> QGMTETISTPAATTTPDLADQQELERRVAQVVSNDPQLQALLPDDAVSGAVNEPGLTLIELIRRLLEGYGDRPALGQRAVELVTDEHGATTVALKTEFVTTSYRELWNRAEAIAAAWYAQGIRDGDFVAQLGFTSTDFASLDVAGLRLGTVSVPLQTGASVQQRNAILEETQPTVFAASVEYLEAAVDSVLATPSVQLLSVFDYHPEADAHRAALSAVRDRLETAGRTITIDSLGDAIARGRELPAAPQPSEDPDALRLLIYTSGSTGTPKGAMYPQWLVANLWQKKWLTTTVIPSVGVNFMPMSHLAGRLTLMGTLSGGGTAYYIASSDLSTFFEDIALIRPTEVLFVPRVVEMVFQRYQAELDRSLAPGESNAEIAEKIKVRIREEDFGGRVLNAGSGSAPLSPEMNDFMESLLQVAMLDGYGSTEAGAVWRDGVLQRPPVTEYKLVDVPELGYFTTDSPHPRGELRIKSETMFPGYYKRPETTADVFDEDGFYMTGDVVAELGPDHLKYLDRVKNVLKLAQGEFVAVSKLEAAYTGSPLVRQIFVYGNSERSYLLAVVVPTPEALERYADSPDALKPLIQDSLQQVAKGAELQSYEIPRDFIVETVPFT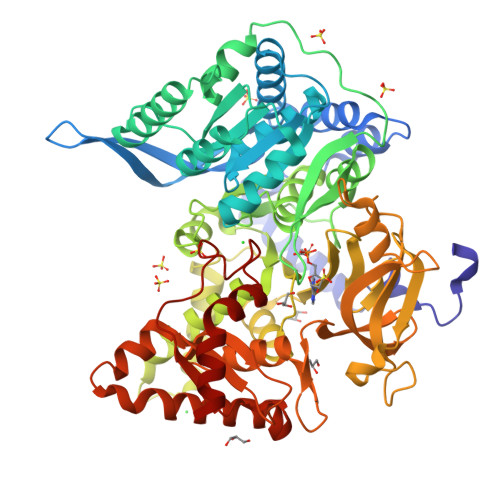VESGLLSDARKLLRPKLKEHYGERLEALYAD>MGSHHHHHHENLYFQGHMNSFYS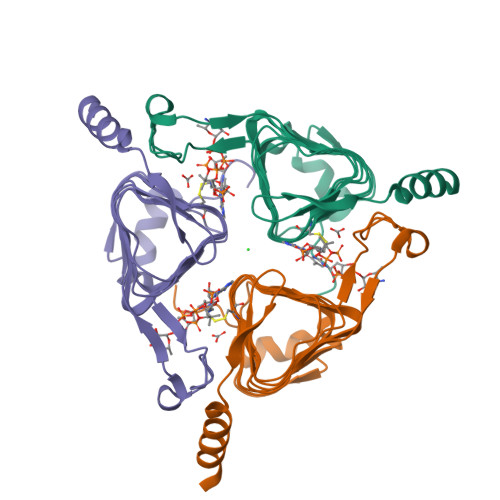QEELKKIGFLSVGKNVLISKKASIYNPGVISIGNNVRIDDFCILSGKVTIGSYSHIAAYTALYGGEVGIEMYDFANICSRTIVYAAIDDFSGNALMGPTIPNQYKNVKTGKVILKKHVIIGAHSIIFPNVVIGEGVAVGAMSMVKESLDDWYIYVGVPVRKIKARKRKIVELENEFLKSMNS[3x]>MKAVQYTEIGSEPVVVDIPTPTPGPGEILLKVTAAGLCHSDIFVMDMPAAQYAYGLPLTLGHEGVGTVAELGEGVTGFGVGDAVAVYGPWGCGACHACARGRENYCTRAADLGITPPGLGSPGSMAEYMIVDSARHLVPIGDLDPVAAAPLTDAGLTPYHAISRVLPLLGPGSTAVVIGVGGLGHVGIQILRAVSAARVIAVDLDDDRLALAREVGADAAVKSGAGAADAIRELTGGQGATAVFDFVGAQST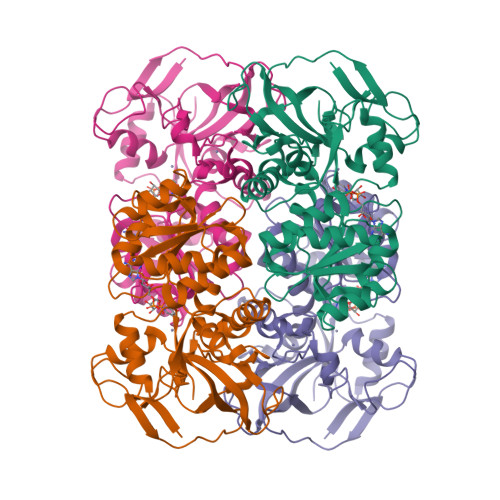IDTAQQVVAVDGHISVVGIHAGAHAKVGFFMIPFGASVVTPFAGTRSELMEVVALARAGRLDIHTETFTLDEGPAAYRRLREGSIRGRGVVVPTSHHHHH[8x]> AAPAVLGEVDTSLVLSSMEEAKQLVDKAYKERRESIKQRLRSGSASPMELLSYFKQPVAATRTAVRAADYLHVALDLLERKLRSLWRRPFNVTDVLTPAQLNVLSKSSGCAYQDVGVTCPEQDKYRTITGMCNNRRSPTLGASNRAFVRWLPAEYEDGFSLPYGWTPGVKRNGFPVALARAVSNEIVRFPTDQLTPDQERSLMFMQWGQLLDHDLDFTPEPAARASFVTGVNCETSCVQQPPCFPLKIPPNDPRIKNQADCIPFFRSCPAC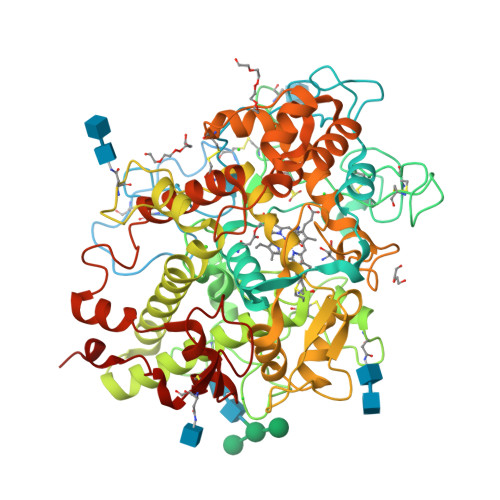PGSNITIRNQINALTSFVDASMVYGSEEPLARNLRNMSNQLGLLAVNQRFQDNGRALLPFDNLHDDPCLLTNRSARIPCFLAGDTRSSEMPELTSMHTLLLREHNRLATELKSLNPRWDGERLYQEARKIVGAMVQIITYRDYLPLVLGPTAMRKYLPTYRSYNDSVDPRIANVFTNAFRYGHTLIQPFMFRLDNRYQPMEPNPRVPLSRVFFASWRVVLEGGIDPILRGLMATPAKLNRQNQIAVDEIRERLFEQVMRIGLDLPALNMQRSRDHGLPGYNAWRRFCGLPQPETVGQLGTVLRNLKLARKLMEQYGTPNNIDIWMGGVSEPLKRKGRVGPLLACIIGTQFRKLRDGDRFWWENEGVFSMQQRQALAQISLPRIICDNTGITTVSKNNIFMSNSYPRDFVNCSTLPALNLASWREAS>MREEQPHLATTWAARGWVEEEGIGSATLGRLVRAWPRRAAVVNKADILDEWADYDTLVPDYPLEIVPFAEHPLFLAAEPHQRQRVL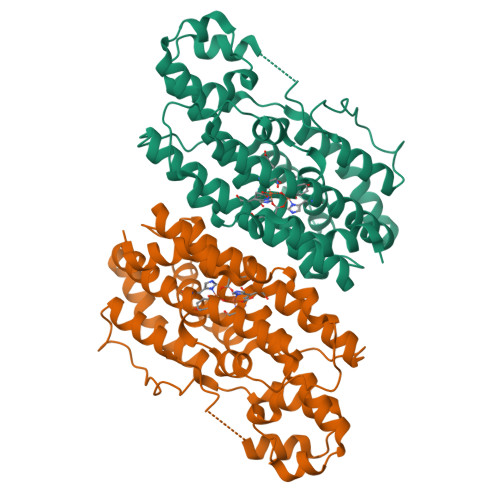TGMWIGYNERVIATEQLIAEPAFDLVMHGVFPGSDDPLIRKSVQQAIVDESFHTYMHMLAIDRTRELRKISERPPQPELVTYRRLRRVLADMPEQWERDIAVLVWGAVAETCINALLALLARDATIQPMHSLITTLHLRDETAHGSIVVEVVRELYARMNEQQRRALVRCLPIALEAFAEQDLSALLLELNAAGIRGAEEIVGDLRSTAGGTRLVRDFSGARKMVEQLGLDDAVDFDFPERPDWSPHTPR[2x]> SMIVRGINMTKIKLESPGFMVHKKLKSMSQSYGVMMTGVPAEVLGQMQAERSIPSINKTGNLKQQIAKEVSKVCHMMTEPTQSCGQASNDVCELLLGKIEAEKFHFTKYEALSADGDNLKNVLENTAPSSTNLLIRFEIDREDPPIVLVKTKNENFNPETAVKNKIYLLENKLYFIDKMGNLFNLGPGKKKCTQLFNAIGDSAEYSLCDPFVLEEPEKPEDFAISEIVDIFNEQKERFDFWIGSHSFTIYIPQTLGESPRQFYPYQAYFGSHTLQDWFVSDKDEYLSRIGIDKYIEKLAVLGKTTNTKERSDIYAEFFSKRGREAFFCAHLNEKRQPLRVKFKITEINPELALKNLQETQEFIDTHPGENPSDKVENYRNRAKLAMTEHLESLLDIKPESS;> SGTFFKDYQKKNVMRLLQDSLEKIINEWLKTDDESHTKLKSLQELSEMDINATSFAEHSPLPDFVTRLWLDPHKALDAMDKNISKNEIRKLIKETAREIELVFTHQK

Strikingly, the SidE- and MavC-type enzymes, two recently identified effector families from the bacterial pathogen Legionella pneumophila, can ubiquitinate host substrates through non-canonical mechanisms without engaging any of the conventional ubiquitination machinery. The genomic cluster of MavC encodes three effector proteins: Lpg2147 (MavC itself), Lpg2148 (MavC paralog A, or MvcA), and Lpg2149. Taken together, our data show that MavC can catalyze deamidation, ubiquitination, and deubiquitination by using the same active pocket. In addition to MavC and MvcA, the same genomic cluster in L. pneumophila also encodes a small effector protein, Lpg2149, which has been shown to interact with both enzymes and inhibit their deamidation activities.

The inhibitory role of Lpg2149 in the MavC system is reminiscent of the function of SidJ in the SidE system, although their operation mechanisms are distinct from each other. To understand the detailed molecular mechanisms of Lpg2149-mediated inhibition, we determined the crystal structures of MavC–Lpg2149 and MvcA–Lpg2149 complexes (X-ray statistics in Table 1). The asymmetric unit contains one Lpg2149 and one enzyme for both structures, highlighting a 1:1 molar ratio of the complex formation. Both structures adopt a similar assembly, with the Lpg2149 monomer binding to the connecting region between Catalytic and HBD domains. Lpg2149 forms similar and extensive hydrogen bonding and hydrophobic interactions with MavC and MvcA, which are mainly mediated by the N-terminal α-helix (aa 11–37) and a helix-loop motif (aa 74–86) of Lpg2149. Upon binding to the enzymes, this C-terminal α-helix folds back and occupies the groove of the very same Lpg2149 molecule. Structural superimpositions between Lpg2149 in its apo and enzyme-bound states show that MavC and MvcA will form heavy steric clashes with the dimeric Lpg2149, thus providing a structural explanation of this dimer-to-monomer conformational transition. However, MvcA undergoes a considerable conformational change by enlarging the relative angle between Catalytic and HBD domains to accommodate Lpg2149, indicating an induced-fit model for MvcA. Isothermal titration calorimetry (ITC) experiments confirm that the binding of Lpg2149–MavC (~0.57 nM) is ~50-fold stronger than that of Lpg2149–MvcA (~28.08 nM). On the other hand, the same set of Lpg2149 mutants show considerable reductions for the inhibition of MvcA-mediated Ub deamidation. Although MvcA shares a high degree of similarity with MavC and possesses Ub-deamidase activity, it cannot catalyze UBE2N ubiquitination.> APNLAGAVEFNDVKTLLRE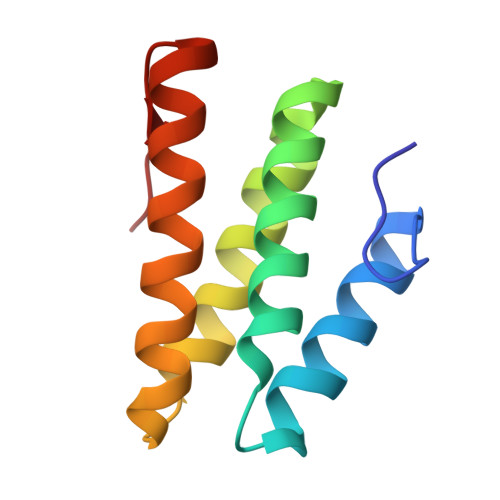WITTISDPMEEDILQVVKYCTDLIEEKDLEKLDLVIKYMKRLMQQSVESVWNMAFDFILDNVQVVLQQTYGSTLKVT> HMFDVVVIGGGISGLSAAKLLTEYGVSVLVLEARDRVGGRTYTIRNEHVDYVDVGGAYVGPTQNRILRLSKELGIETYKVNVSERLVQYVKGKTYPFRGAFPPVWNPIAYLDYNNLWRTIDNMGKEIPTDAPWEAQHADKWDKMTMKELIDKICWTKTARRFAYLFVNINVTSEPHEVSALWFLWYVKQCGGTTRIFSVTNGGQERKFVGGSGQVSER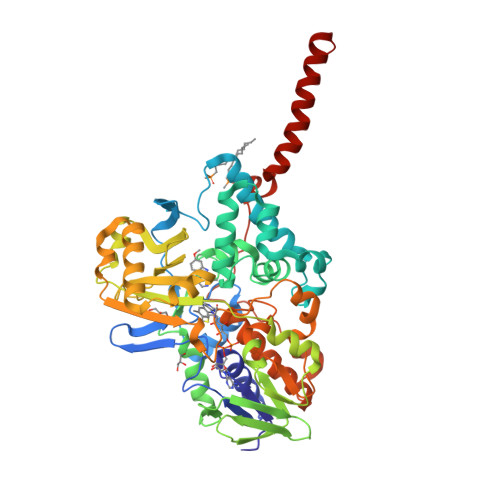IMDLLGDQVKLNHPVTHVDQSSDNIIIETLNHEHYECKYVINAIPPTLTAKIHFRPELPAERNQLIQRLPMGAVIKCMMYYKEAFWKKKDYCGCMIIEDEDAPISITLDDTKPDGSLPAIMGFILARKADRLAKLHKEIRKKKICELYAKVLGSQEALHPVHYEEKNWCEEQYSGGCYTAYFPPGIMTQYGRVIRQPVGRIFFAGTETATKWSGYMEGAVEAGERAAREVLNGLGKVTEKDIWVQEPESKDVPAVEITHTFWERNLPSVSGLLKIIGFSTSVTALGFVLYKYKLL>[4x]AMKKDSKAPCVEVFDERDGCKAAGTQKASGDDGFCVKVS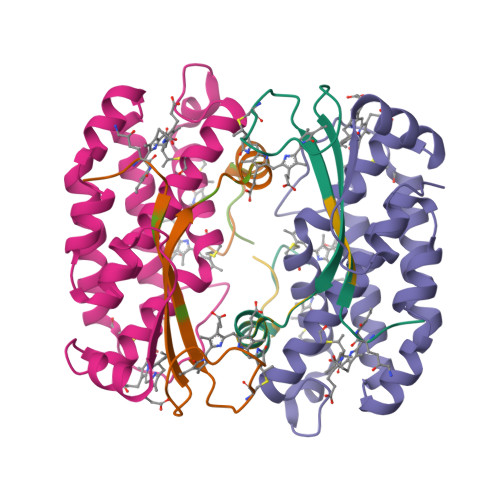MKAIGFNAAEAASVTKNYGIKRFGAKSV;>MLDAFSKVITSADGKAAYVGGADLQALKKFVSEGNKRMDSVNAIVSNASCIVSDSVSGMVCENPSLIAPNGGVYTNRKMAACLRDAEIILRYVSYSLLSGDSSVLEDRCLNGLKETYASLGVPAAGNARTISIMKATVIGFITNNSQQKKLSTPAGDCSALASEVGGYFDKVSSALA[4x];>AMKKDSKAPCVEVFDERDGCKAAGTQKASGDDGFCVKVSMKAIKMNAAEATSVTKNYNTKLL[4x]The enzyme N-myristoyltransferase (NMT) is one of only a few genetically and chemically validated drug targets in kinetoplastids, with the NMT inhibitor DDD85646 being shown to act on target and to cure the mouse model of stage-1 (non-CNS) T. brucei infection.[5–8] Functionally the NMT enzyme is ubiquitous and is responsible for catalysing the co-translational transfer of myristate from myristoyl-CoA to the N-terminal glycine residue of the target protein. Work was initially carried out without X-ray co-crystal structures; when this structural information was established using the Leishmania major enzyme, key early-stage molecules were also co-crystallised with the enzyme. As we discussed in a previous publication, the L. major NMT shows high sequence homology to both the T. brucei and human NMTs. Compounds around two different cores, thiazolidinones and benzomorpholinones, were validated as hits for TbNMT.

Simultaneous replacement of the R1 3-phenol-4-methoxy groups of 1 with a 2-pyridyl unit, and truncation of the R2 benzyl group to a directly linked phenyl, resulted in compound 7 and an unexpected inversion of the binding mode from that observed for 6, giving rise to binding mode T2. Compounds that adopted binding mode T2 show the R1 2-pyridyl subunit forming a hydrogen bonding interaction with the side chain of Ser330, and the thiazolidinone carbonyl group forming a hydrogen bonding interaction with the side chain of Asn376. The X-ray crystal structure also revealed the R2 substituent to be located in the hydrophobic peptide binding groove, lying in a similar plane to the aryl group in the pyrazole sulfonamide series. In binding mode T2, and in contrast to 6, the S enantiomer was bound in the active site. It is unclear why compound 7 displayed selectivity for TbNMT over hNMT. However, this observed selectivity was lost upon removal of the (R2-phenyl)-3-chloro substituent, seen with 9, although this is partly due to the overall diminished potency observed for this compound. Substitution at the ortho or meta positions of the R2 phenyl group appeared to be preferred over para substitution which may be due to a clash of this substituent with the side chain of Tyr217. Interestingly, the thiazolidinone compounds displayed two distinct binding modes with different enantiomers bound.

> MGSSHHHHHHSSGRENLYFQGPSNSDAAHAFWSTQPVPQTEDETEKIVFAGPMDEPKTVADIPEEPYPIASTFEWWTPNMEAADDIHAIYELLRDNYVEDDDSMFRFNYSEEFLQWALCPPNYIPDWHVAVRRKADKKLLAFIAGVPVTLRMGTPKYMKVKAQEKGEGEEAAKYDEPRHICEINFLCVHKQLREKRLAPILIKEATRRVNRTNVWQAVYTAGVLLPTPYASGQYFHRSLNPEKLVEIRFSGIPAQYQKFQNPMAMLKRNYQLPSAPKNSGLREMKPSDVPQVRRILMNYLDSFDVGPVFSDAEISHYLLPRDGVVFTYVVENDKKVTDFFSFYRIPSTVIGNSNYNLLNAAYVHYYAATSIPLHQLILDLLIVAHSRGFDVCNMVEILDNRSFVEQLKFGAGDGHLRYYFYNWAYPKIKPSQVALVML>[2x]MTEKGRAIEEESFRIVDQEAGPHGFSPLEWPVVRRMIHATADFEYKALTRFSQGAVEAGLKA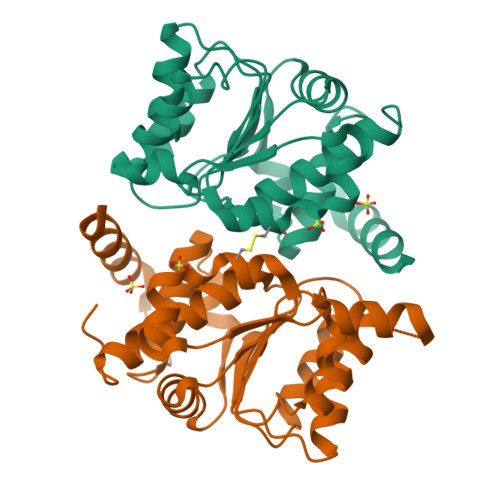IQAGARILVDARMIACGLNPERLRLFGNEVVELLAHPEVVARAKATGGTRAEAAVAYAWEKGLLDGAIVGVGNAPTFLLALVEAIRQGARPALVLGMPVGFVNVLEAKRALMEAPVPWIVTEGRKGGSTLVVAALHALIRLAADGGVDTSRAYREG> SMGAVMGTFSSLQTKQRRPSKDIAWWYYQYQRDKIEDELEMTMVCHRPEGLEQLEAQTNFTKRELQVLYRGFKNECPSGVVNEDTFKQIYAQFFPHGDASTYAHYLFNAFDTTQTGSVKFEDFVTALSILLRGTVHEKLRWTFNLYDINKDGYINKEEMMDIVKAIYDMMGKYTYPVLKEDTPRQHVDVFFQKM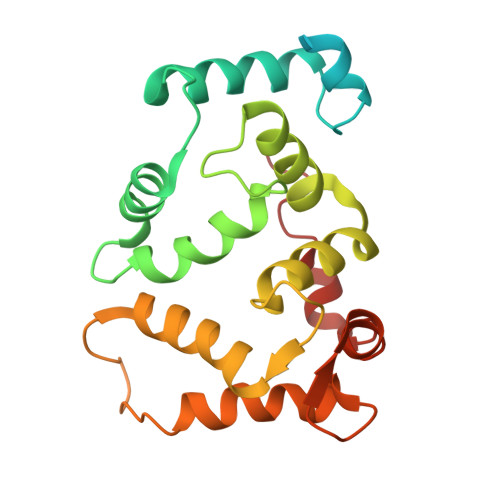DKNKDGIVTLDEFLESCQEDDNIMRSLQLFQNVM>[8x]MSADYPRDLIGYGNNPPHPHWPGDARIALSFVLNYEEGGERCVLHGDKESEAFLSEMVAAQPLQGVRHMSMESLYEYGSR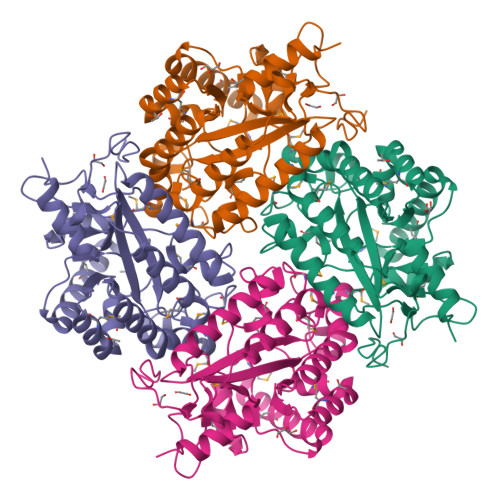AGVWRLLKLFKRRNVPLTVFAVAMAAQRNPEVIRAMVADGHEICSHGYRWIDYQYMDEAQEREHMLEAIRILTELTGQRPVGWYTGRTGPNTRRLVMEEGGFLYDSDTYDDDLPYWDPASTAEKPHLVIPYTLDTNDMRFTQVQGFNNGEQFFQYLKDAFDVLYEEGATAPKMLSIGLHCRLIGRPARMAALERFIQYAQSHDKVWFARREDIARHWHREHPFQETEA>MSSQKVFGITGPVSTVGATAAENKLNDSLIQELKKEGSFETEQETANRVQVLKILQELAQRFVYEVSKKKNMSDGMARDAGGKIFTYGSYRLGVHGPGSDIDTLVVVPKHVTREDFFTVFDSLLRERKELDEIAPVPDAFVPIIKIKFSGISIDLICARLDQPQVPLSLTLSDKNLLRNLDEKDLRALNGTRVTDEILELVPKPNVFRIALRAIKLWAQRRAVYANIFGFPGGVAWAMLVARICQLYPNACSAVILNRFFIILSEWNWPQP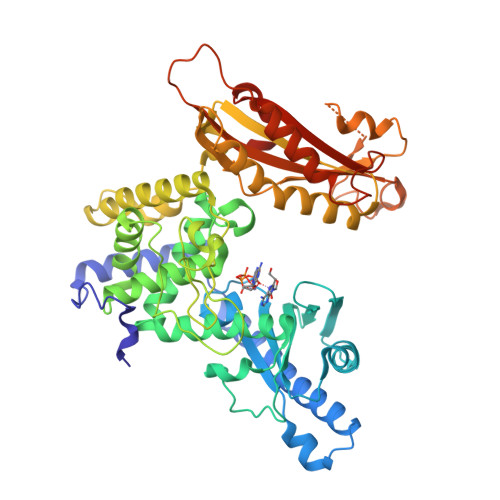VILKPIEDGPLQVRVWNPKIYAQDRSHRMPVITPAYPSMCATHNITESTKKVILQEFVRGVQITNDIFSNKKSWANLFEKNDFFFRYKFYLEITAYTRGSDEQHLKWSGLVESKVRLLVMKLEVLAGIKIAHPFTKPFESSYCCPTEDDYEMIQDKYGSHKTETALNALKLVTDENKEEESIKDAPKAYLSTMYIGLDFNIENKKEKVDIHIPCTEFVNLCRSFNEDYGDHKVFNLALRFVKGYDLPDEVFDENEKRPSKKSKRKN[2x]> GGSLTEQDRQLRLLQAQIQR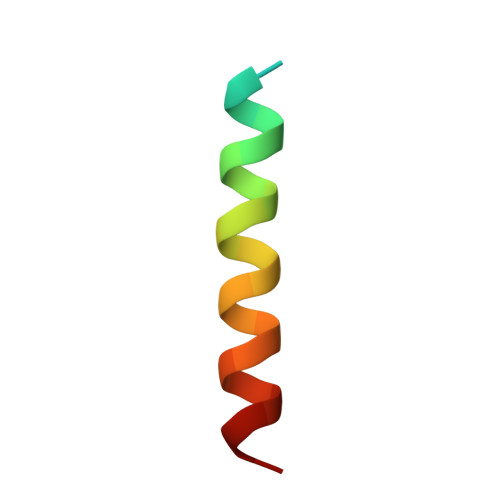LLEAQSLM> MELHQIRGCHKNDIELKKYNIGVAISLGNKWFSIDNIEKLVKWSLLHTKEYVIIYIADSIHGINLSVRNKLSDSHAEEVAIRYGRNLFIKIKERVSLSFSQDEQAKIIYATWSDIADSKYKEKVKYLYNLYDKNINFKNYIENFVKEWVSKEKRTFNNNEINKFGRYILEELPELMVQVKARGVLFEAFVYPYKTRITEFVGLLQKGEIFPEIKTNILD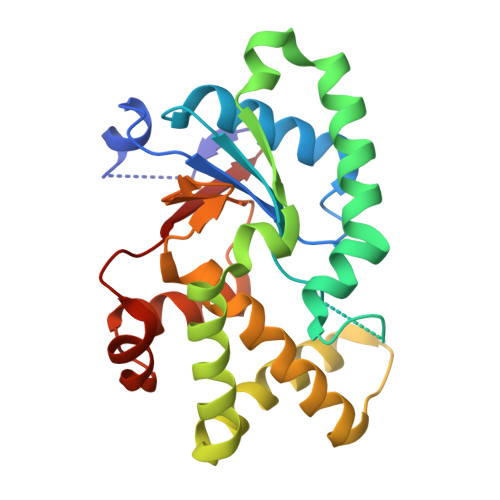NHPKIFLEVRE> SQD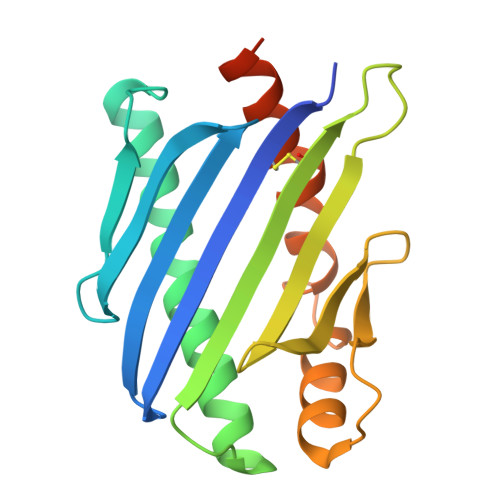ASDGLQRLHMLQISYFRDPYHVWYQGNASLGGHLTHVLEGPDTNTTIIQLQPLQEPESWARTQSGLQSYLLQFHGLVRLVHQERTLAFPLTIRCFLGCELPPEGSRAHVFFEVAVNGSSFVSFRPERALWQADTQVTSGVVTFTLQQLNAYNRTRYELREFLEDTCVQYVQKHISAENTKGSQTSRSYTS>MQAHEESQLMRISATINGKPRVFYVEPRMHLADALREVVGLTGTKIGCEQGVCGSCTILIDGAPMRSCLTLAVQAEGCSIETVEGLSQGEKLNALQD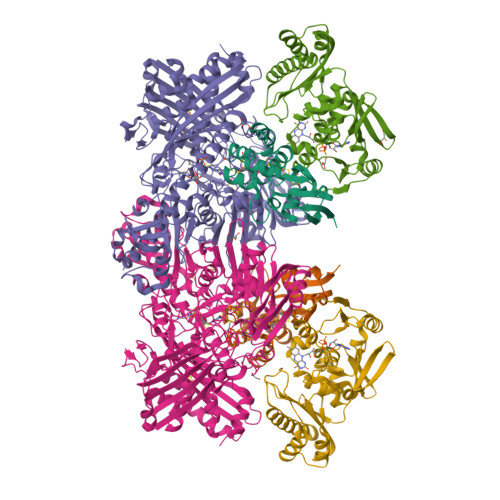SFRRHHALQCGFCTAGMLATARSILAENPAPSRDEVREVMSGNLCRCTGYETIIDAITDPAVAEAARRGEV[2x];>[2x]MMKHEVVALKKKSIGTSVLRREDTRLLTGRGRYIADLVLSGMLHVASLRSPFAHARIVSIDVADAQALPGVELVWCGADVAELSQGIVATMQVEGFQTTIQPLLANGVTRFVGEIVAVVVASSRAIAEDAAQLIQVEYEELPAVTGIEAALEGEARANDTLAGNVVSRTSRARDELAPIFASSAGVVRGQFSCGRVSACPMETRGAVAQYEWTTQQLILWTATQMPSFVRTMVAMFCAIPEHLIEVRVPDVGGGFGQKAHLHPEELLVCLLSRALGRPVRWIEDRQENFLGATHAKQQRNEMGLAFDGDGRFLALENRSITDGGAYNNLPWTQLVESHVGNAVILGVYKVPAVSEESIAVATNKCPIGAYRGVGFTAGQIARETLIDRAARQLGLSPFEIRRRNVVMPEDFPFTNRLGQTHREGTYLQTINLLEEMVNPEAFRQRQAEARARGKYLGLGVSVFNEVTGTGTRTLSFLGTPTTTHDSATVRIDPTGKVTVTTSLASSGQGHETTLAQIAADVLGVPASDVVIQAGSTKNTYGFGAYASRGAVIGAGSIGRAASIVRERVKQLAGHLLEAASEDIVIEDGLVHVAGVPAKGMPFAEVVGAAYFADATHPPGFDATLEATATYDPSDLVLANGGHAAIVEIDASTYATRVTDFFAVEDCGTMINPMIVEGQIRGGIAQAIGQTLLEEVIYDDFGQLVTTTLMDYLIPTTLDVPDIRIRHLETPSPLVPGGIKGMGESAMISAPAAVVAAVNDALAHLEVVIETVPITPERIFRSIQERPMQ;>[2x]MKFPAFSYRAPASLQEVIQVLADDPDARIIAGGQSLLPLLAFRLVYPSCLVDLRNVSELFEISQSAGILSVGAMVTHFRNKTDPTVAKCVPILPKVLAHVAHQAVRNRGTLGGSLAHADAGAEMPFLMATLGATMYIASSAGVRSVSATDFMKGHYFTDLEAGEVLVRVEIPIPALHWEFDEYARRKGDYALVMAAAGLSMQGGRCVAARIALGAVEERAHQAIRANDFLVGKVIDESTAATAAELATEGLEPRSDIHGSRDLRLSLAKAITQRVILKAAQGAMYAGA>[2x]ATSLEKHVLLKKLRDALESLRGR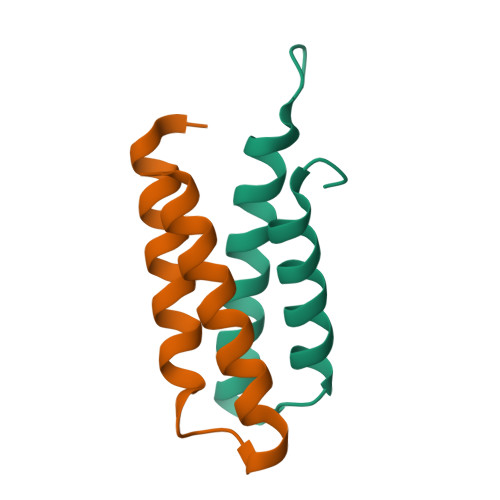VAGRNKDDVEEAIAMVEALAVQLTQREGE> ALVKEEIQAKEYLENLNKELAKRTNVETEAAWAYGSNITDENEKKKNEISAELAKFMKEVASDTTKFQWRSYQSEDLKRQFKALTKLGYAALPEDDYAELLDTLSAMESNFAKVKVCDYKDSTKCDLALDPEIEEVISKSRDHEELAYYWREFYDKAGTAVRSQFERYVELNTKAAKLNNFTSGAEAWLDEYEDDTFEQQLEDIFADIRPLYQQIHGYVRFRLRKHYGDAVVSETGPIPMHLLGNMWAQQWSEIADIVSPFPEKPLVDVSAEMEKQGYTPLKMFQMGDDFFTSMNLTKLPQDFWDKSIIEKPTDGRDLVCHASAWDFYLTDDVRIKQCTRVTQDQLFTVHHELGHIQYFLQYQHQPFVYRTGANPGFHEAVGDVL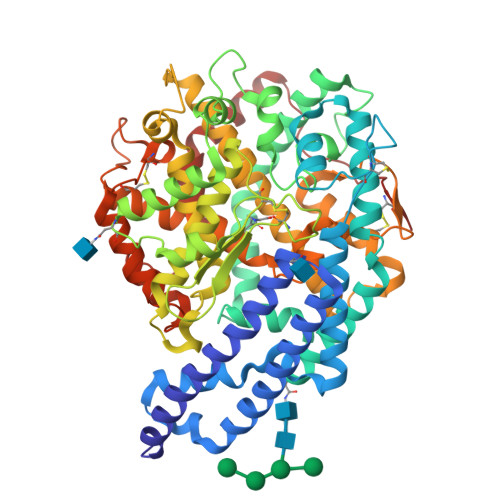SLSVSTPKHLEKIGLLKDYVRDDEARINQLFLTALDKIVFLPFAFTMDKYRWSLFRGEVDKANWNCAFWKLRDEYSGIEPPVVRSEKDFDAPAKYHISADVEYLRYLVSFIIQFQFYKSACIKAGQYDPDNVELPLDNCDIYGSAAAGAAFHNMLSMGASKPWPDALEAFNGERIMSGKAIAEYFEPLRVWLEAENIKNNVHIGWTTSNKCVS>MQQSVCRARPIWWGTQRRGSETMAGAAVKYLSQEEAQAVDQELFNEYQFSVDQLMELAGLSCATAIAKAYPPTSMSK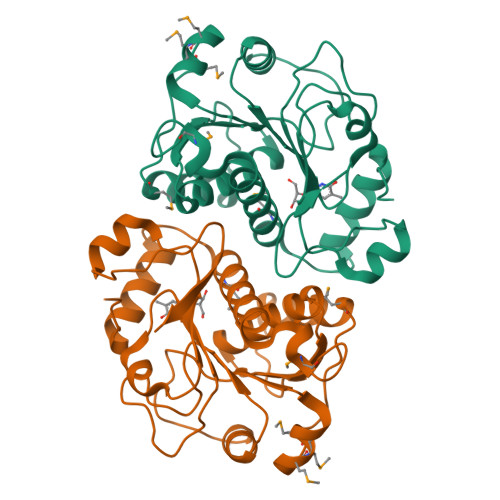SPPTVLVICGPGNNGGDGLVCARHLKLFGYQPTIYYPKRPNKPLFTGLVTQCQKMDIPFLGEMPPEPMMVDELYELVVDAIFGFSFKGDVREPFHSILSVLSGLTVPIASIDIPSGWDVEKGNPSGIQPDLLISLTAPKKSATHFTGRYHYLGGRFVPPALEKKYQLNLPSYPDTECVYRLQHHHHHH[6x]> MAQPSQSSVPESDAGSFPVDIHKPFTPAERIQQLGEIDNDI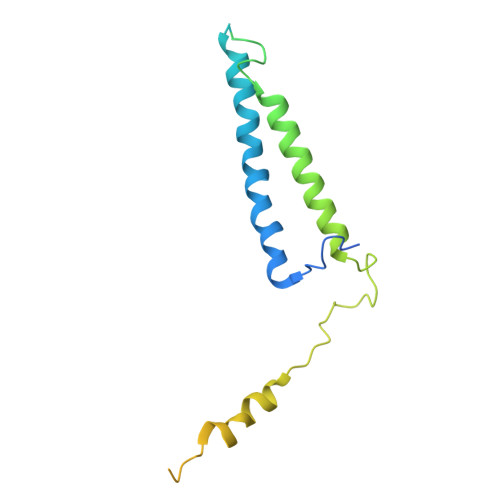ASLLQHLSAALKALATPPGKRIFQEQDSESNSPSASDTSNPNDTPPSSCGIDPVTAFKTAQNDFFRTIDRIDKHLTRQIYALEEAGIITLKSGTGSGAGTVGAGATEEQAQQLPQPQMIPGQPQAAGITADASVAPVPKARLEPDGMGRYGKLDVGRLNMASSIVEREMEGELWRKAREHLGRMTSQASGREDRMEE>LQKSIGHKPEPTDEEWELIKTVTEAHVATNAQGSHWKQKRKFLPEDIGQAPIVNAPEGGKVDLEAFSHFTKIITPAITRVVDFAKKLPMFCELPCEDQIILLKGCCMEIMSLRAAVRYDPESETLTLNGEMAVTRGQLKNGGLGVVSDAIFDLGMSLSSFNLDDTEVALLQAVLLMSSDRPGLA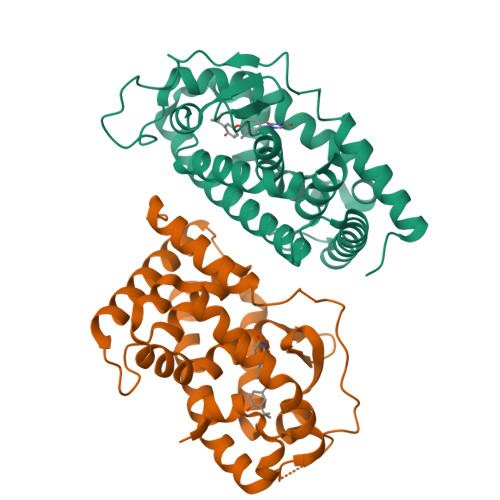CVERIEKYQDSFLLAFEHYINYRKHHVTHFWPKLLMKVTDLRMIGACHASRFLHMKVECPTELFPPLFLEVFED[2x]> TPVAEETRARLSKELQAAQARLGADMEDVCGRLVQYRGEVQAMLGQSTEELRVRLASHLRKLRKRLLRDADDLQKRLAV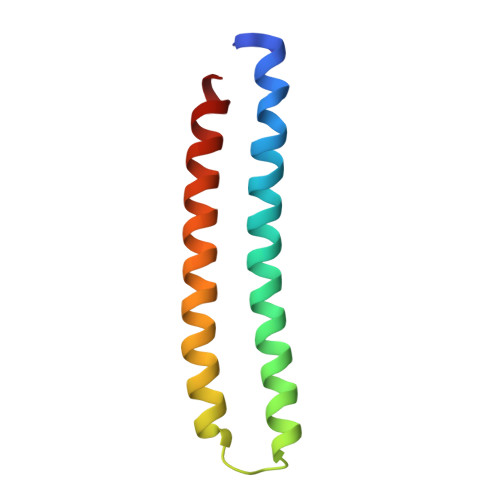YQAG> MALCKFCDVRFSTCDNQKSCMSNCSITSICEKP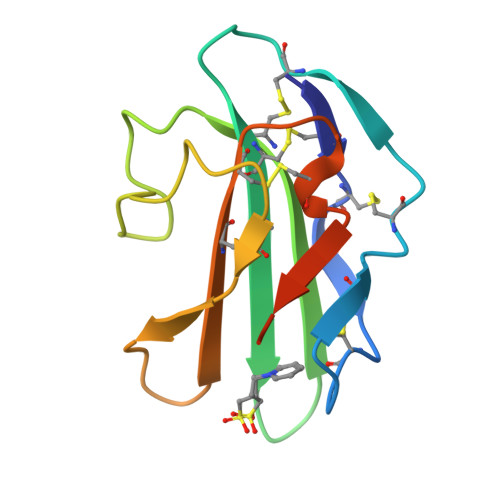QEVCVAVWRKNDENITLETVCHDPKLPYHDFILEDAASPTCIMKEKKKPGETFFMCSCSSDECNDNIIFSEEYNTSNPD> GAMVLTQTHATGHVGDFFFTHWKDGGSTSLTLDAEGKFLVTWQGGGYNYVGGPGWHFGDKNRVIRYKLNEETGASYIALYGWGYDKTMSESDPSHLVEYYILQRWTYDPSQDGIYGKTFVSNGIEYSTYRSIRKVKPSINGPTTFYQYWSKPSAQQELGKDHKIIFADHVKAWADTGWILPDMNNFDASDDPTYQVLAVEVFNPQKNGTASGQVWDE

A number of predicted genes that showed similarity to carbohydrate active enzymes (CAZymes) were selected for expression leading to the discovery of the first exo-1,4-β-xylanase from glycoside hydrolase family 11 (GH11). This enzyme was able to degrade xylooligomers, which are known inhibitors to commercially available cellulase cocktails, as well as xylan, yielding xylobiose as the only reaction product. The protein compost21_GH11 was predicted as a GH11 family member and shared 77% identity with a non-characterized GH from Marinimicrobium agarilyticum. Compost21_GH11 was found to be an exo-1,4-β-xylanase with highest activity against xylan at pH 6.0 at 35 °C. The enzyme retained more than 60% activity for all tested pHs, but the observed activity quickly dropped at temperatures higher than 40 °C. However, at 35 °C and pH 6.0, compost21_GH11 retained 90% activity for up to 96 h.

In order to understand the molecular basis of exo-1,4-β-xylanase activity, the crystal structure of compost21_GH11 was solved at 1.76 Å resolution. The final model was constructed from the first to last residue of the crystallized protein, which was cloned without the first 13 residues that were predicted as a disordered region and reported as a signal peptide. The structure of compost21_GH11 shows a typical GH11 fold of a β-jelly-roll. The curvature of the β-sheets B1 to B9 forms a cleft where the catalytic residues (nucleophile Glu98 in β-sheet B6 and proton donor Glu200 in β-sheet B4) are located. Two extra loops (EL1 and EL2) are found in the compost21_GH11 structure. They are created by additional residues, which stretch between β-sheets B5 and B6 and in β-sheet B4, respectively. EL2 blocks substrate interaction at subsite − 3, which accommodates the non-reducing end of xylan. This loop is stabilized by a number of hydrogen bonds within the loop main/side chain residues and van der Walls interactions, especially between Pro192 and Phe186 side chains. Hydrogen bonds are also established with EL1 and with the turn that connects β-sheets B7 and B8. Here, we show that loop EL2 blocks one side of compost21_GH11 active site, transforming this enzyme into an exo-1,4-β-xylanase that acts from the non-reducing end.> TLEDDYANAWQEWS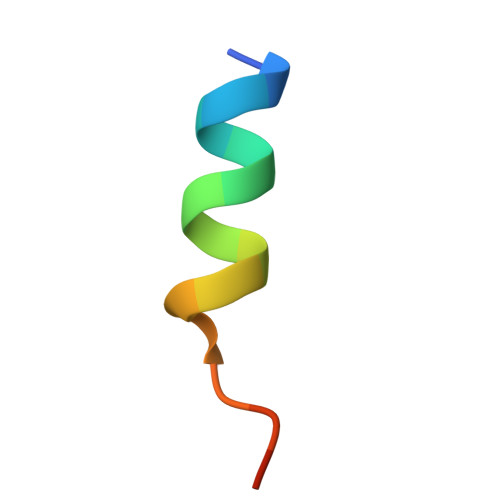AAG>PMFIVNTNVPRASVPDGFLSELTQQLAQATGKPPQYIAVHVVPDQLMAFGGSSEPCALCSLASIGKIGGAQNRSYSKLLCGLLAERLRISPDRVYINYYDMNAANVGWNNSTFA[3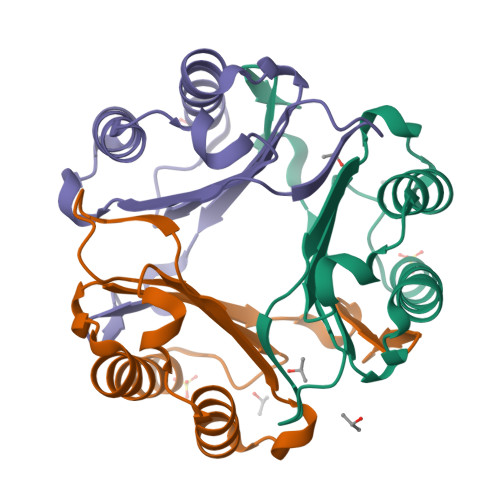x]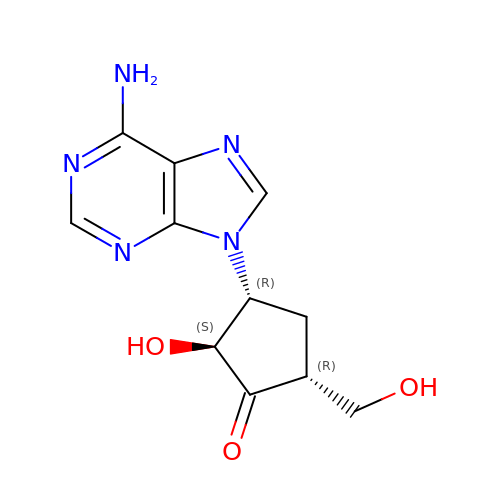(2S,3R,5R)-3-(6-amino-9H-purin-9-yl)-2-hydroxy-5-(hydroxymethyl)cyclopentanone | C11 H13 N5 O3 | CWNCBQJCRSRXGI-KCRUCZTKSA-N> SMAQKLNLLNLAVPPVTHRSNFPSTFTFGVATSAYQIEGGWNEGKKGPSIWDKFTHIEGKILDGSNGDVAVDHYHRYKEDVDLIGQLGFGAYRFSISWSRIFPDGLGTEVNEEGIAFYNDLINTLLEKGIQPYVTLYHWDLPSHLQEAIGGWTNRKIVDYFGLYADACFANFGDRVKHWITLNEPLQTSVNGHCIGIFAPGRNEKPLIEPYLVSHHQVLAHATAVSIYRSKYKESQGGQIGLSVDCEWAEPNSEKPEDKVAADRRIDFQLGW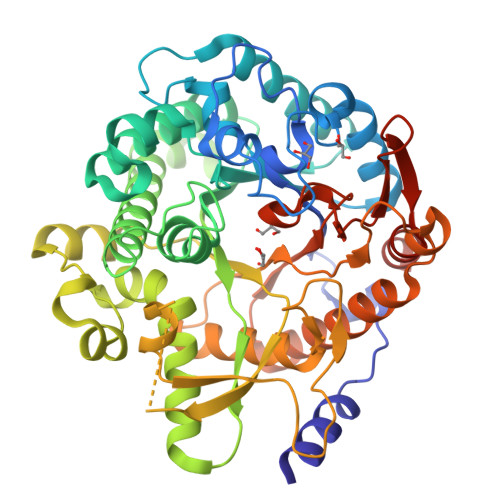FLDPLFFGDYPASMRQKLGDNLPRFTPEEKEFMLQNSWDFLGLNHYTSRLISHVSNKEAESNFYQAQELERIVELENGDLIGERAASDWLYAVPWGIRKTLNYMSKKYNHPPIFITENGMDDEDDGSASIHDMLDDKRRVDYFKSYLANVSQAIEDGVDIKGYFAWSLLDNFEWAQGYTKRFGLVYVDYKNGLTRHPKSSAYWFMKFLKGDEENKGKKE>MSQNQVPKWIQLNNEIMIQKDGKFQFDKDKEAVHSYFVDYINQNTVFFHNLKEKLDYLVENQYYEEEFLSLYSFEDIKEVFKTAYAKKFRFPSFMSAFKFYNDYALKTNDKKKILERYEDRISIVALFFANGDTEKAKEYVNLMINQEYQPSTPTFLNAGRKRRGELVSCFLLEVNDSLNDISRAIDISMQLSKLGGGVSLNLSKLRAKGEAIKDVENATKGVVGVMKLLDNAFRYADQMGQRQGSGAAYLNIFHRDINDFLDTKKISADEDVRVKTLSIGVVIPDKFVELAREDKAAYVFYPHTIYKEYGQHMDEMDMNEMYDKFVDNPRVKKEKINPRKLLEKLAMLRSESGYPYIMFQDNVNKVHANNHISKVKFSNLCSEVLQASQVSSYTDYDEEDEIGLDISCNLGSLNILNVMEHKSIEKTVKLATDSLTHVSETTDIRNAPAVRRANKAMKSIGLGAMNLHGYLAQNGIAYESPEARDFANTFFMMVNFYSIQRSAEIAKEKGET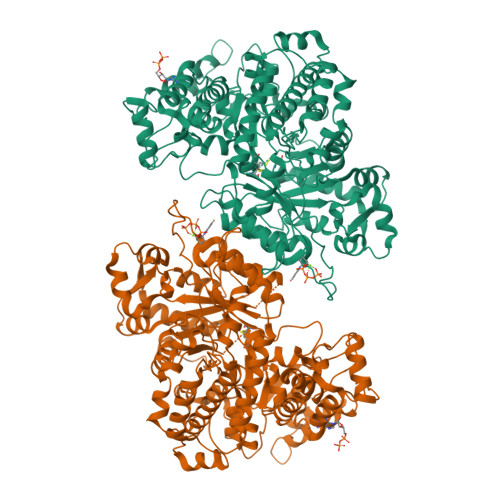FDQYEGSTYATGEYFDKYVSTDFSPKYEKIANLFEGMHIPTTEDWKKLKAFVAEHGMYHSYRLCIAPTGSISYVQSSTASVMPIMERIEERTYGNSKTYYPMPGLASNNWFFYKEAYDMDMFKVVDMIATIQQHIDQGISFTLFLKDTMTTRDLNRIDLYAHHRGIKTIYYARTKDTGQDSCLSCVV[2x]ADP-ribosyl-L-arginine 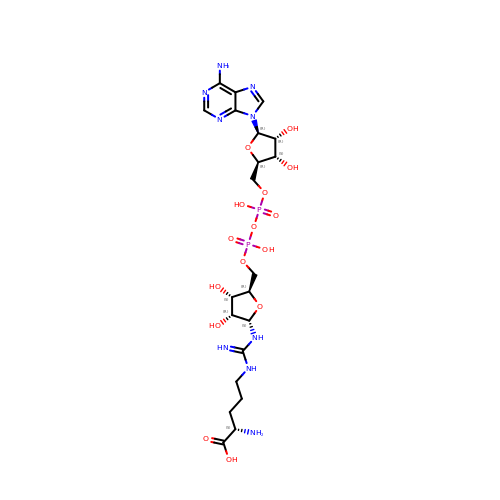| C21 H35 N9 O15 P2 | IWVSYNGKNZFSSA-PTDVUUCPSA-N>[2x]ESQ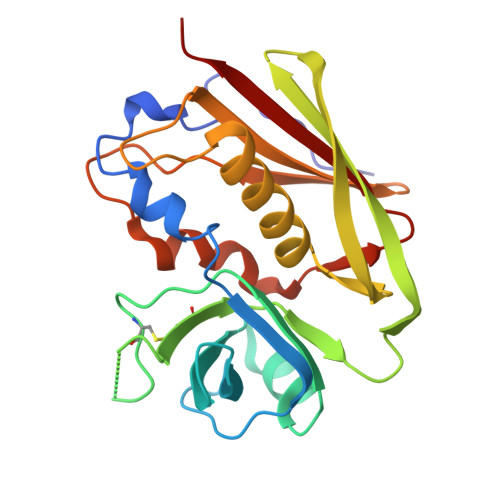PDPKPDELHKSSKFTGLMENMKVLYDDNHVSAINVKSIDQFLYFDLIYSIKDTKLGNYDNVRVEFKNKDLADKYKDKYVDVFGANYYYQCYFSKKTNDINSHQTDKRKSCMYGGVTEHNGNQLDKYRSITVRVFEDGKNLLSFDVQTNKKKVTAQELDYLTRHYLVKNKKLYEFNNSPYETGYIKFIENENSFWYDMMPAPGDKFDQSKYLMMYNDNKMVDSKDVKIEVYLTTKKK>MNHKVHHHHHHIEGRHMEEHYYVSIDIGSSSVKTIVGEKFHNGINVIGTGQTYTSGIKNGLIDDFDIARQAIKDTIKKASIASGVDIKEVFLKLPIIGTEVYDESNEIDFYEDTEINGSHIEKVLEGIREKNDVQETEVINVFPIRFIVDKENEVSDPKELIARHSLKVEAGVIAIQKSILINMIKCVEACGVDVLDVYSDAYNYGSILTATEKELGACVIDIGEDVTQVAFYERGELVDADSIEMAGRDITDDIAQGLNTSYETAEKVKHQYGHAFYDSASDQDIFTVEQVDSDETVQYTQKDLSDFIEARVEEIFFEVFDVLQDLGLTKVNGGFIVTGGSA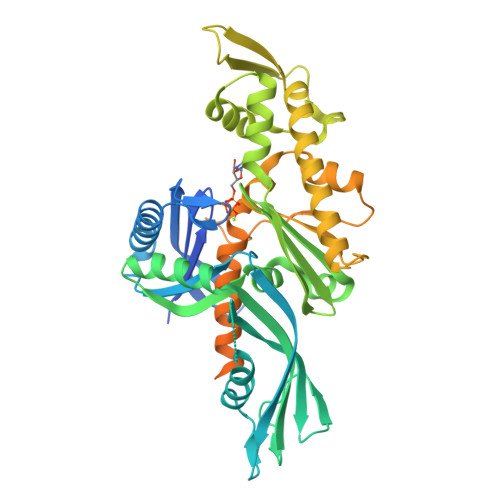NLLGVKELLSDMVSEKVRIHTPSQMGIRKPEFSSAISTISSSIAFDELLDYVTINYHDNEETEEDVIDVKDKDNESKLGGFDWFKRKTNKKDTHENEVESSDEEIYQSEDNHQEHKQNHEHVQDKDKEESKFKKLMKSLFE[4x]> MNSNIPNSPDERIQNHGGDEQHNGDHNERNNPYFARQQASAEPDLDANEPILRSSDIKRLNRKALVFLAAIAALLILAIFWLATQSGEDSAPPKPRTETVVAPALPQSMTAPVEEAPVPLAQQPSLPPLPPMPTDNSEEVSSAPERQRGPTLLERRILAESAANGGGVPGQLGAQPAPTQEDGPVTLAKPISNPDGLL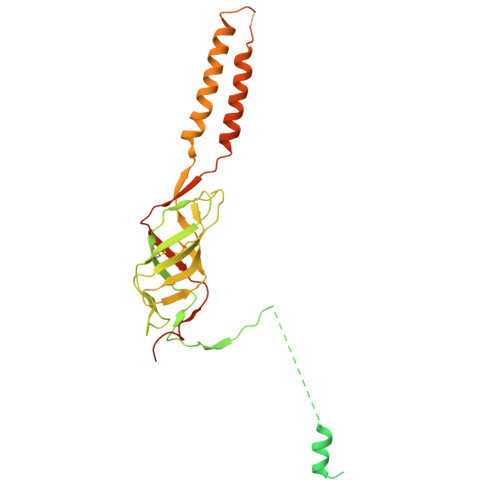VRGTYIRCILETRIISDFGGYTSCIVTEPVYSINGHNLLLPKGSKMLGQYSAGEPTSHRLQVVWDRVTTPTGLDVTLMGPGIDTLGSSGHPGNYNAHWGNKIASALFISLLSDAFKYAAAEYGPETTTIGVGSGIVTQQPFESNTARSMQQLAEQAVEKSGRRPATLTINQGTVLNVYVAKDVDFSAVLPKAAALEGLSAWSHPQFEK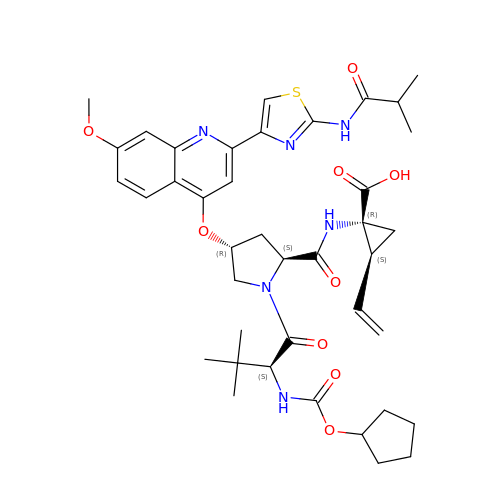N-[(cyclopentyloxy)carbonyl]-3-methyl-L-valyl-(4R)-N-[(1R,2S)-1-carboxy-2-ethenylcyclopropyl]-4-[(7-methoxy-2-{2-[(2-methylpropanoyl)amino]-1,3-thiazol-4-yl}quinolin-4-yl)oxy]-L-prolinamide | C40 H50 N6 O9 S | GEXHIQCMKLNKQH-LONKKFHASA-N> GAMGSFNSIDVEINMYPVNKTSCNSSIGSSSTISTSELTITLTHEDCTPVFIGDYYSVVDKLATSGFFTNDKVHQDLTTQCKINLEIKCNSGRESRQLTPTTKVYLMPHSETVTVVGDCLSNLDVYIVYANTDAIYSDMDVVAYHTSYILNVDHIPPNDCERD;> GAMGQHHGVTKCNITCSKMTSKIPVALLIHYQQNQASCGKRAIILETRQHRLFCADPKEQWVKDAMQHLDRQAAALTRNG

In addition to the anti-TNF activity attributed to the N-terminal four cysteine-rich domains (CRDs) homologous to host TNF receptors, CrmB and CrmD have anti-chemokine activity attributed to a unique C-terminal extension (∼160 aa), named as the SECRET domain (smallpox virus-encoded chemokine receptor). Biochemical analysis revealed that the SECRET domain binds a subset of human and mouse CC, CXC and C chemokines, including CCL28, CCL25, CCL20, CXCL12, CXCL13, CXCL14, and XCL1. The identification of other poxvirus genes encoding homologues with the SECRET domain indicates that the SECRET domain represents a new family of viral CKBPs, which has specific folding to allow its binding with chemokines, either independently or fused with vTNFRs. Here we report the crystal structures of the SECRET domain of CrmD encoded by an ECTV strain and the complex of it with chemokine CX3CL1.

To directly elucidate the chemokine binding by the SECRET domain, we reconstituted a complex of the SECRET domain with the chemokine domain of CX3CL1 and determined its structure at a resolution of 2.6 Å. In the complex, one SECRET domain monomer binds one CX3CL1 monomer, displaying a 1∶1 stoichiometry. The SECRET domain contacts the CX3CL1 with its β-sheet I, burying a surface of ∼530 Å2. The SECRET domain contacting residues are from the strands 1, 5, and 6 of β-sheet I and the C-terminal extended loop, while the CX3CL1 contacting residues are from the N-loop, 310 helix, 40s loop, and the β3 strand. The binding interface can be described as a small hydrophobic core surrounded by a large halo of hydrophilic interactions. The hydrophobic core is composed of residues Y212 and F225 from CrmD, and I19, L23 and F49 from CX3CL1. The acidic residues D167, E169, and D316 from the SECRET domain form salt-bridge interactions with R44, R47, and K18 from CX3CL1, respectively. Mutating charged residues K18, R44, and R47 in CX3CL1 induced more significant binding affinity decrease than mutating hydrophobic residues I19, L23, and F49, suggesting the importance of the salt-bridge interactions in the complex formation of the SECRET domain with CX3CL1. The SECRET domain utilizes its β-sheet I to interact with CX3CL1, whereas vCCI utilizes its β-sheet II to interact with CCL4 upon complex formation. It suggests that although the SECRET domain does not directly block the most important receptor binding site on CX3CL1 (i.e. the N-termini and critical hydrophobic residues of the N-loop), its binding is still close to the receptor binding site and bring steric hindrance to prevent efficient interaction with the receptor, which would provide a structural basis for the ability of the SECRET domain to inhibit CX3CL1 and CCL25 induced cell migration.>SNFFVIKAKENGVNVFGMTRGTDTRFHHSEKLDKGEVMIAQFTE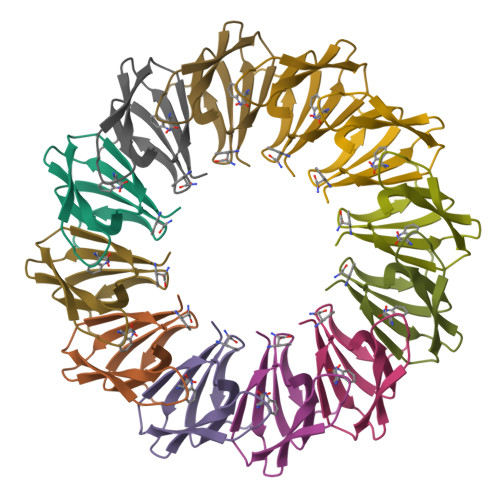HTSAVKIRGKAIIQTSYGTLDTEKDE[3x]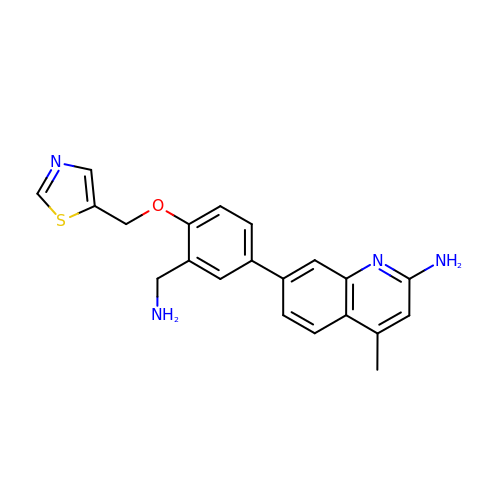7-{3-(aminomethyl)-4-[(1,3-thiazol-5-yl)methoxy]phenyl}-4-methylquinolin-2-amine | C21 H20 N4 O S | SHBUNLMNTXCFTE-UHFFFAOYSA-N> MAAAPFISLLQGDQFLADTPIPGSAVIPNSGNLFPKWADKLSPTAVETWLFDAMAEDGSAAFTVSFFRDGSQAPASFRAAINAAWSDGTVWSQHLVVPVSVVTSDGPDVGHGHVAGVWRTEEPQSNDTTRTTASFDVAADLSTTTVVFDAPGRITGSLTHRSLGYPTLPQSDREAEVAPGAYWFRPIAMANATVD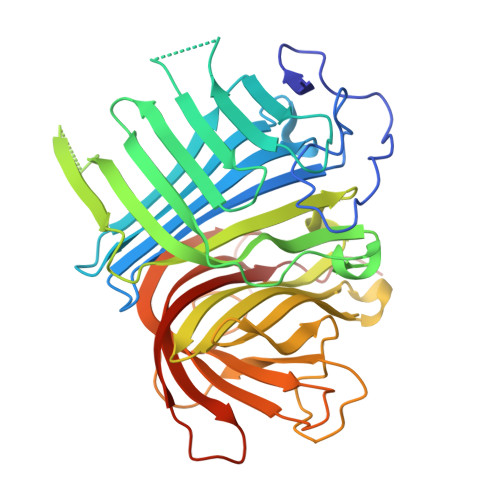LTFHIDDPTNPDKKTEKRMVLGPEQGAFGGMDRSWLPMVWGKEATDALFVRAQAGPYVMAVMRLVSKPHKYYQNTVNAALYRDGKIVSNALRSLPPDRRDTAATADAVRTEKLYDGDGLVAKYRDKNVGYRLEFRSAGPEREKWSFDLRHHQAWWAKPTSRPGPDGTGNSGFVVEVTGGLVGSEESVHGWGMTGEVELSDGHHHHHHHHH>[2x]MAPSAGEDKHSSAKRVAVIGAGVSGLAAAYKLKIHGLNVTVFEAEGKAGGKLRSVSQDGLIWDEGANTMTESEGDVTFLIDSLGLREKQQFPLSQNKRYIARNGTPVLLPSNPIDLI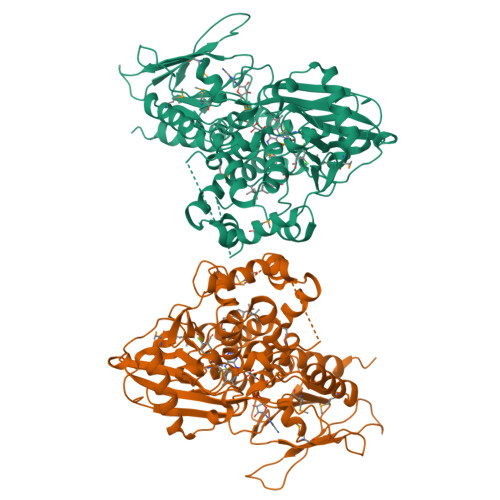KSNFLSTGSKLQMLLEPILWKNKKLSQVSDSHESVSGFFQRHFGKEVVDYLIDPFVAGTCGGDPDSLSMHHSFPELWNLEKRFGSVILGAIRSKLSPKNEKKQGPPKTSANKKRQRGSFSFLGGMQTLTDAICKDLREDELRLNSRVLELSCSCTEDSAIDSWSIISASPHKRQSEEESFDAVIMTAPLCDVKSMKIAKRGNPFLLNFIPEVDYVPLSVVITTFKRENVKYPLEGFGVLVPSKEQQHGLKTLGTLFSSMMFPDRAPNNVYLYTTFVGGSRNRELAKASRTELKEIVTSDLKQLLGAEGEPTYVNHLYWSKAFPLYGHNYDSVLDAIDKMEKNLPGLFYAGNHRGGLSVGKALSSGCNAADLVISYLESVSTDSKRHC> LTFDLPFEELLTYPGRTPRPADHDEYWDRGLADLAAVPADVVIEPAEFTTPLARCSHLWFTGTGGVRVHAKLLRPVAPVEPHPALLQFHGYTGNSGDWSSRLHYVALGYTVAALDCRGQAGLSVGEAPVENWSMASYLLRGIDDDAADNLALRHLFLDTARLAQIVL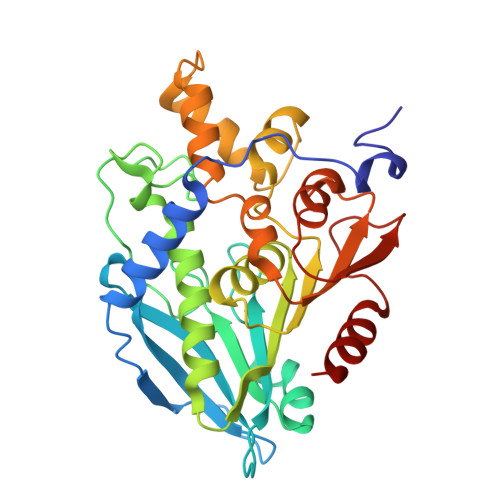AMDDVDPDRVAATGYSQGGGLTLACAALEPRIRLAAPVYPFLCDFRRAWEMDLEKGPYNEITTYFRARDPRHLREEEIFSRLGYVDVQHLAPRVRAEVLMTVSLADKICPPSTQFAAYNKLGGPKDYRLYPDFAHETLPGTDDAIFTFLQGL> H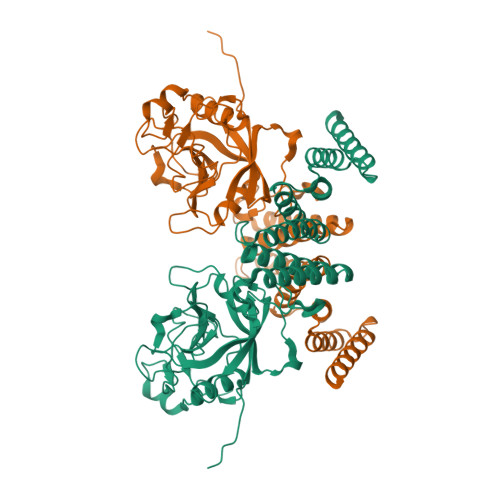HHMMIQDPLVYLDISIDKKPIGRIVCKLFREKAPKTTENFYKLCAGDVKSPLKDQQYLSYKGNGFHRVVKNFMIQAGDIVFGTQKDSSSSSVGKGGCSIYADKEEVKTDDESFCYGNFEDENLGEFVEPFTLGMANLGSPNTNNSQFFITTYAAPHLNGKHSIFGQVVHGKSVVRTIENCRVDSDGVPESDVRISDCGVWEKTMGVPLYNASNDQIGGDVYEEYPDDDTHFGDDDFGKALEAANIIKESGTLLFKKKDYSNAFFKYRKSLNYINEYMPEPDVDKERNIQFINLKMKIYLNLSLVLFNLERYDDAIMYATYLLEMDNVPNRDQAKAYYRRGNSYLKKKRLDEALQDYIFCKEKNPDDEVIEQRIEYVNRLIEENKEKTRKNISKFFS> MQGVRYIYHHFYTSLLVFVVMILFRSALSIYINTLSSTESLTISNNRTLVSPGDVFELGFFTPGSSSRWYLGIWYKKLSERTYVWVANRDNPLSNSTGTLKISGNNLVLRGDSNKS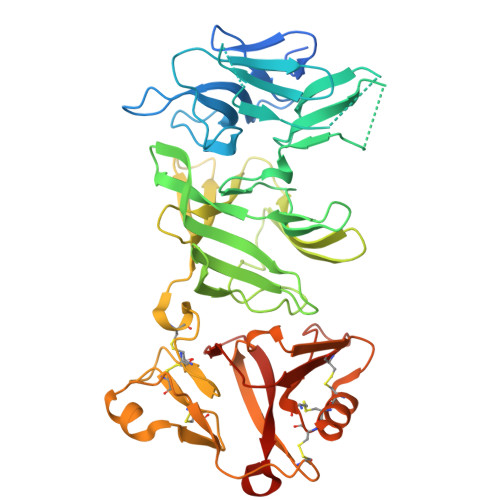IWSTNLTRGNERSPVVAELLANGNFVMRDSNNNDASGFLWQSFDYPTDTLLPEMKLGYDLKTGRNRFLTSSRNSDDPSSGDYSYKLEPRRLPEFYLLQGDVREHRSGPWNGIQFSGIPEDQKSSYMVYNFTENSEEVAYTFRMTNNSFYSRLTINSEGYLERLTWAPSSGAWNVFWSSPNHQCDMYRMCGPYSYCDVNTSPSCNCIQGFNPGNVQQWALRNQISGCKRRTRLSCNGDGFTRMKNIKLPDTRMAIVDRSIGLKECEKRCLSDCNCTAFANADIRNRVTGCVIWTGELEDMRNYAEGGQDLYVRLAAADSRLEVLFQGP2',3'-DIDEOXY-3'-FLUORO-URIDIDINE-5'-DIPHOSPHATE | C9 H13 F N2 O10 P2 | 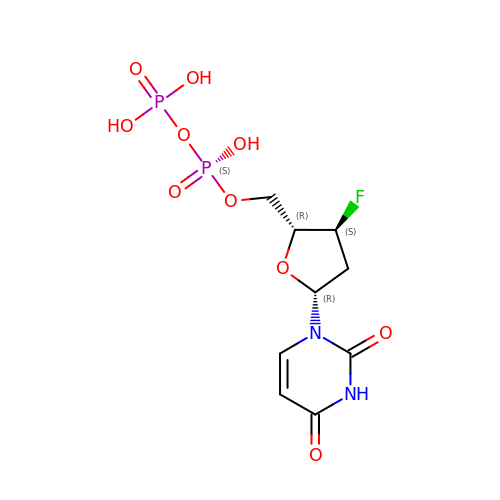WLQBZMZTRNPUDL-SHYZEUOFSA-N>AEKEDRGRPYTLSVALPGSILDNAQSPELRTYLAGQIARACAIFCVDEIVVFDEEGQDAKTVEGEFTGVGKKGQACVQLARILQYLECPQYLRKAFFPKHQDLQFAGLLNPLDSPHHM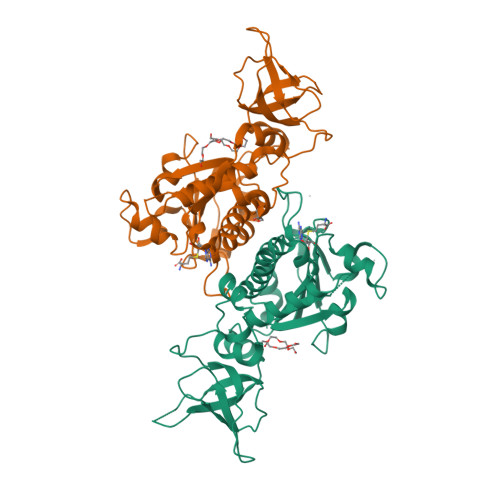RQDEESEFREGIVVDRPTRPGHGSFVNCGMKKEVKIDKNLEPGLRVTVRLNQQQHPDCKTYHGKVVSSQDPRTKAGLYWGYTVRLASCLSAVFAEAPFQDGYDLTIGTSERGSDVASAQLPNFRHALVVFGGLQGLEAGADADPNLEVAEPSVLFDLYVNTCPGQGSRTIRTEEAILISLAALQPGLTQAGARHT[2x]> MITSALHRAADWAKSVFSSAALGDPRRTARLVNVAAQLAKYSGKSITISSEGSKAAQEGAYRFIRNPNVSAEAIRKAGAMQTVKLAQEFPELLAIEDTTSLSYRHQVAEELGKLGSIQKASRGWWVHSVLLLEATTFRTVGLLHQEWWMRPDDPADADEKESGKWLAAAATSRLRMGSMMSNVIAVCDREADIHAYLQDKLAHNERFVVRSKHPRKDVESGLYLYDHLKNQPELGGYQISIPQKGVVDKRGKRKNRPARKASLSLRSGRITLKQGNITLNAVLAEEINPPKGETPLKWLLLTSEPVESLAQALRVIDIYTHRWRIEEFHKAWKTGAGAERQRMEKPDN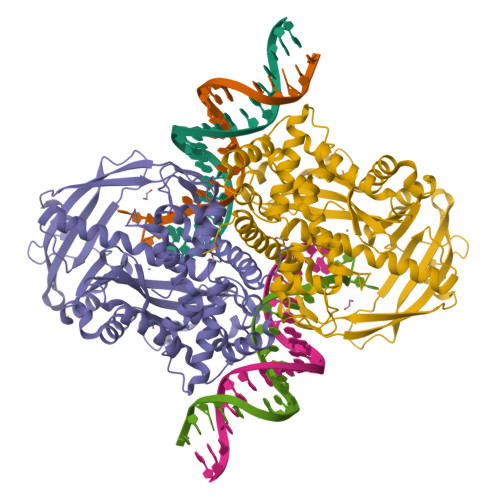LERMVSILSFVAVRLLQLRESFTPPQALRAQGLLKEAEHVESQSAETVLTPDECQLLGYLDKGKRKRKEKAGSLQWAYMAIARLGGFMDSKRTGIASWGALWEGWEALQSKLDGFLAAKDLMAQGIKIG> MDVVSLDKPFMYFEEIDNELDYEPESANEVAKKLPYQGQLKLLLGELFFLSKLQRHGILDGATVVYIGSAPGTHIRYLRDHFYNLGVIIKWMLIDGRHHDPILNGLRDVTLVTRFVDEEYLRSIKKQLHPSKIILISDVASAAGGNEPSTADLLSNYALQNVMISILNPVASSLKWRCPFPDQWIKDFYIPHGNKMLQPFAPSYSAEMRLLSIYTGENMRLTRVTKSDAVNYEKKMYYLNKIVRNKVVVNFDYPNQEYDYFHMYFMLRTVYCNKTFPTTKAKVLFLQQSIFRFLNIP;> MNRNPDQNTLPNITLKIIETYLGRVPSVNEYHMLKSQARNIQKITVFNKDIFVSLVKKNKKRFFSDVNTSASEIKDRILSYFSKQTQTYNIGKLFTIIELQSVLVTTYTDILGVLTIKAPNVISSKISYNVTSMEELARDMLNSMNVAVIDKAKVMGRHNVSSLVKNVNKLMEEYLRRHNKSCICYGSYSLYLINPNIRYGDIDILQTNSRTFLIDL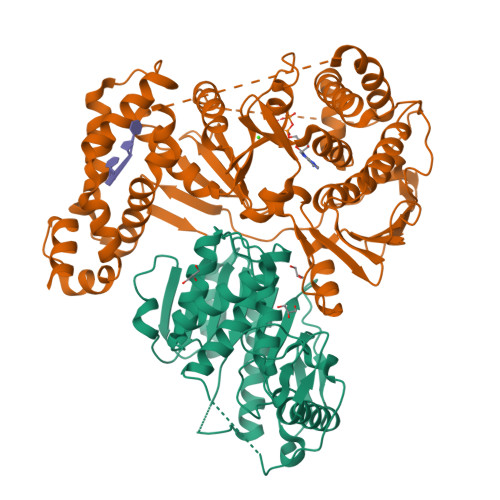AFLIKFITGNNIILSKIPYLRNYMVIKDENDNHIIDSFNIRQDTMNVVPKIFIDNIYIVDPTFQLLNMIKMFSQIDRLEDLSKDPEKFNARMATMLEYVRYTHGIVFDGKRNNMPMKCIIDENNRIVTVTTKDYFSFKKCLVYLDENVLSSDILDLNADTSCDFESVTNSVYLIHDNIMYTYFSNTILLSDKGKVHEISARGLCAHILLYQMLTSGEYKQCLSDLLNSMMNRDKIPIYSHTERDKKPGRHGFINIEKDIIVF> MEIMDEIKVNLQKEVSLEEAERYAKNIASKYGDGILLSV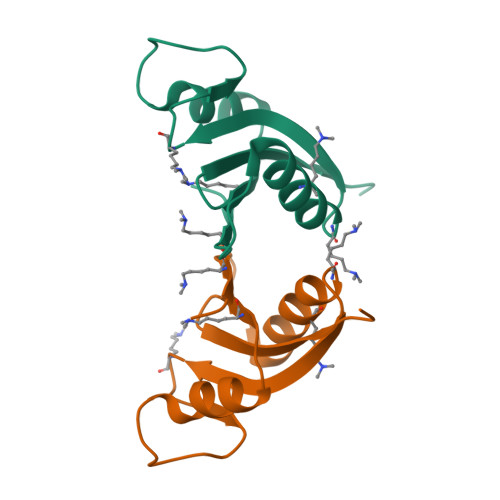HDSKTGYRAPEVYCCGEKPWEVYACNRGANLKISVNQFEFYFRIEVEGQAKY>[4x]MDKFRVQGPTKLQGEVTISGAKNAALPILFAALLAEEPVEIQNVPKLKDVDTSMKLLSQLGAKVERDGSVHIDARDVNVFCAPYDLVKTMRASIWALGPLVARFGQGQVSLPGGCTIGARPVDLHISGLEQLGATIKLEEGYVKASV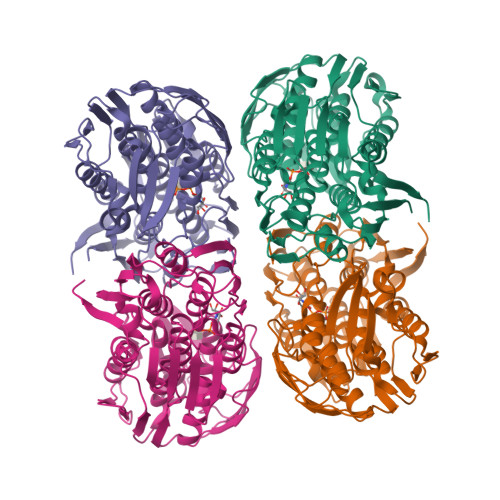DGRLKGAHIVMDKVSVGATVTIMCAATLAEGTTIIENAAREPEIVDTANFLITLGAKISGQGTDRIVIEGVERLGGGVYRVLPDRIETGTFLVAAAISRGKIICRNAQPDTLDAVLAKLRDAGADIEVGEDWISLDMHGKRPKAVNVRTAPHPAFPTDMQAQFTLLNLVAEGTGFITETVFENRFMHVPELSRMGAHAEIESNTVICHGVEKLSGAQVMATDLRASASLVLAGCIAEGTTVVDRIYHIDRGYERIEDKLRALGANIERVKGELVPR Here, we expand the repertoire of known macromolecular biotin binders by reporting a novel biotin-binding protein A (BBP-A) from chicken. In the present study, we show that the chicken BBP-A gene encodes a functional homotetrameric protein. The BBP-A structures consist of four identical subunits, each subunit adopting a β-barrel fold of eight anti-parallel β-strands with an α-helix positioned between the β7- and β8-strands. The BTN/BSO-binding site is located at the open end of each β-barrel.

In order to study the molecular details of ligand recognition by BBP-A and compare the ligand-binding properties of BBP-A with the previously determined structures of AVD, streptavidin, AVR4 and AVR2, we crystallized bBBP-A in complex with BTN. The crystal structures of bBBP-A in complex with BTN and BSO were solved at 2.1 Å and 1.75 Å resolution, respectively. The biotin-binding site of the BBP-A – BTN structure mimics the biotin-binding site of AVD. The amino acid residues within 4 Å of BTN in the complex with BBP-A (Asn12, Leu14, Ser16, Tyr33, Thr35, Val37, Thr38, Ala39, Thr40, Trp71, Phe73, Ala74, Ser76, Thr78, Phe80, Trp98, Leu100, Glu102, Asn119 and Trp111) are not only highly conserved but also have conformations similar to those seen in AVD. The side-chain oxygen of Glu102 of BBP-A is hydrogen bonded to one of the valeric oxygen atoms of BTN, whereas in AVD the equivalent residue, Ser101, can not form a hydrogen bond to the valeric oxygen because the distance between the two atoms is too long (5.8 Å). The methyl carbon of Ala74 of BBP-A, on the other hand, is positioned only 3.7 Å away from the valeric O10B atom of BTN (numbering according to [26]), but is not likely to be hydrogen bonded with BTN unlike the side-chain oxygen atom of the corresponding Ser73 in AVD, which is hydrogen bonded to BTN. One clear difference can, however, be detected: the hydrogen bond present in the BBP-A – BTN complex structure between Glu102 and BTN is missing in the BBP-A – BSO structure due to the different conformation of Glu102 in the two structures. The binding mode of BTN to BBP-A is also highly similar to that observed in the known structures of AVD, AVR2 and AVR4. The overall BBP-A – BTN and BBP-A – BSO structures are practically identical to each other; the Cα atoms of these structures superimpose with an rmsd of < 0.2 Å. The BBP-A protein binds free biotin with high, "streptavidin-like" affinity (Kd ~ 10-13 M), which is about 50 times lower than that of chicken avidin.

> GTRKCELQGLWRNELGSNMTISALDVAGTFSGSYQTAVTATNKQILVSPLKGAQQPPGTKGQQPTFGFTVQWQFADSTTVFVGQCFVDRRGKEMLEMAWLLREEVPSRKDTWKATRVGTNVFTRVK> MPPRPSSGELWGIHLMPPRILVECLLPNGMIVTLECLREATLITIKHELFKEAR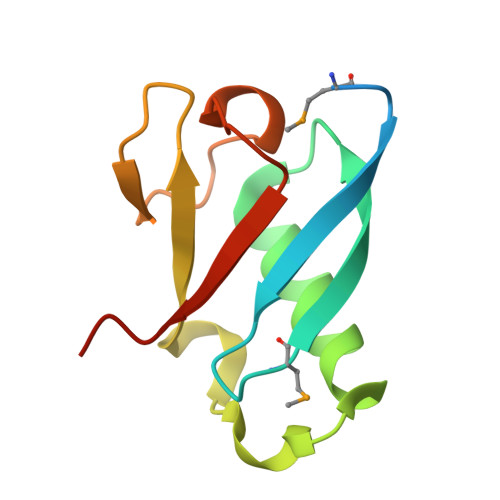KYPLHQLLQDESSYIFVSVTQEAEREEFFDETRRLCDLRLFQPFLKVIEPVGNR>GASTAQPKQEAYIQSTELFLQNKYSDVITTLEDYAPEDMPYVIQYELASSYVMTESLTEEQRQTVSNN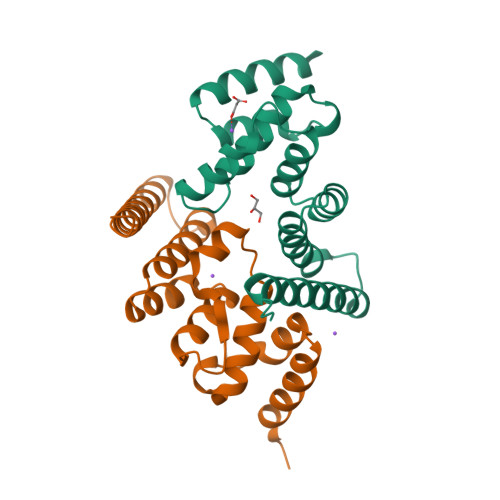ITLKTDEQYMLYWIYIGRSQSEEALELARTIEDRDLIVYALLKYREQIKGDTDLSGDEKQKKLDEIDQEIKEYERERKESEAQLEEEQQSEQQ[4x]propan-2-yl hydrogen 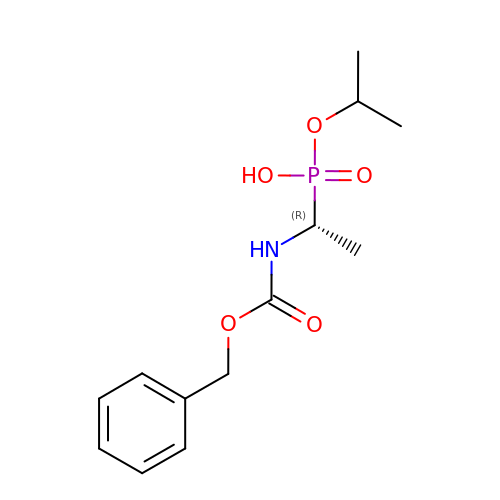(S)-[(1R)-1-{[(benzyloxy)carbonyl]amino}ethyl]phosphonate | C13 H20 N O5 P | DRLKMEFBZYZZJV-LLVKDONJSA-N>[2x]MGHMMSNAEAFYASIRTELESIRAAGLFKNERVIATPQGARVRTTDGREVINLCANNYLGLSSHPQVIEAAHEALRTHGFGLSSVRFICGTQDLHKTLEARLSAFLGTEDTILYGSAFDANGGLFETLLGAEDAVISDALNHASIIDGVRLSKARRYRYQHNDMDDLRVQLEQARADGARYTLVFSDGVFSMDGTVARLDEMRAICDEYGALLGIDECHATGFMGQRGRGTHEA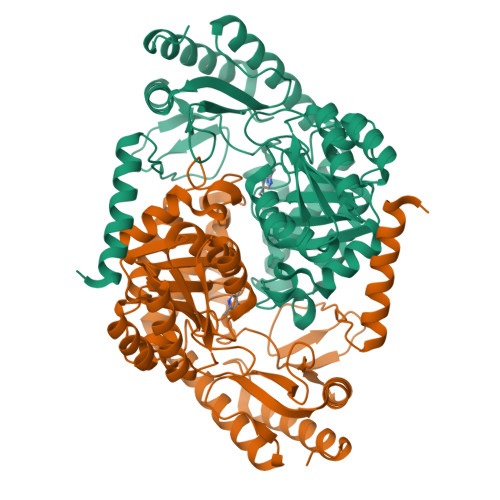RGVFGKIDIITGTLGKALGGASGGFTSARKEVVALLRQRSRPYLFSNTVAPAIVGASIAVLDILEASTELRDRLEGNTRFFRAGLDRLGFDVKAGDHPIIPIMVYDADKAQQLAQRLLELGVYVVGFFYPVVPKGQARIRVQMSALHDEAALQAALDAFGQAGRELGLILEHHHHHH>[18x]MSVLTIGDKRLGAALLDAGLLTDEELQRALERHREVGGSLAEVLVDMGLLSERRIAQTIEDRFGIPLVELHRVEIPPKVKALLPAEKAKELKAIPFALDEEAGVVRVAFLNPLDTLSLEEVEDLTGLVVEPYQTTKSAFLYALAKHYPELGLPVPPPPSGEGQKDLKLGELLLQKGWISREALEEALVEQEKTGDLLGRILVRKGLPEEALYRALAEQKGLEFLESTEGIVPDPSAALLLLRSDALRYGAVPIGFQNGEVEVVLSDPRHKEAVAQLLNRPARFYLALPQAWEELFRRAYPQKNRLGEVLVQEGKLSREALKEALEVQKGLPRAKPLGEILVELGLARPEDVEEALQKQRRGGGRLEDTLVQSGKLRPEALAQAVATQLGYPYVDPEEDPPDPGAPLLLPEDLCRRYGVFPHRLEGNRLVLLMKDPRNILALDDVRL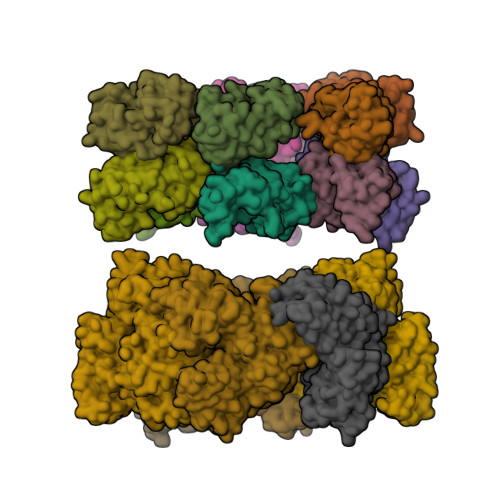ALKRKGLNYEVAPAVATEAAITKLIERFYGKAELSEIAKEFAKKQAEEEVPSPLELDESAAQKFVKQVIREAFLQDASDIHIEPRQNDVQVRLRIDGALRPYSTLPKGALNAVISVVKIMGGLNIAEKRLPQDGRVRYREGAIDVDLRLSTLPTVYGEKAVMRLLKKASDIPEIEDLGFAPGVFERFKEVISKPYGIFLITGPTGSGKSFTTFSILKRIATPDKNTQTIEDPVEYEIPGINQTQVNPQAGLTFARALRAFLRQDPDIIMVGEIRDSETAKIATEAALTGHLVIATLHTNDAAQAITRLDEMGVEPFNISAALIGVLSQRLVRRVCEHCKVEVKPDPETLRRLGLSEAEIQGARLYKGMGCERCGGTGYKGRYAIHELLVVDDEIRHAIVAGKSATEIKEIARRKGMKTLREDGLYKALQGITTLEEVLARTIEAAAELALVPRGSSAHHHHHHHHHH> FNLDAEAPAVLSGPPGSFFGFSVEFYRPGTDGVSVLVGAPKANTSQPGVLQGGAVYLCPWGASPTQCTPIEFDSKGSRLLESSLSSSEGEEPVEYKSLQWFGATVRAHGSSILACAPLYSWRTEKEPLSDPVGTCYLSTDNFTRILEYAPCRSDFSWAAGQGYCQGGFSAEFTKTGRVVLGGPGSYFWQGQILSATQEQIAESYYPEYLINLVQGQLQTRQASSIYDDSYLG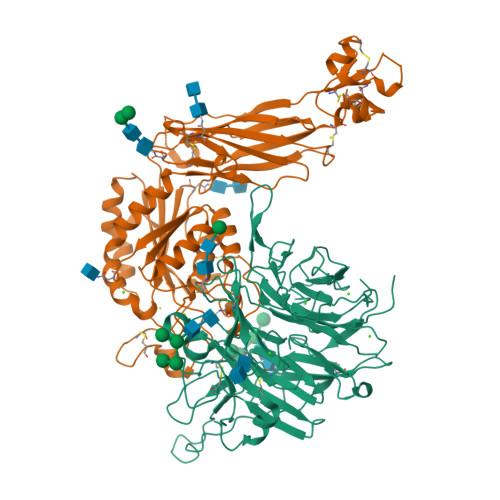YSVAVGEFSGDDTEDFVAGVPKGNLTYGYVTILNGSDIRSLYNFSGEQMASYFGYAVAATDVNGDGLDDLLVGAPLLMDRTPDGRPQEVGRVYVYLQHPAGIEPTPTLTLTGHDEFGRFGSSLTPLGDLDQDGYNDVAIGAPFGGETQQGVVFVFPGGPGGLGSKPSQVLQPLWAASHTPDFFGSALRGGRDLDGNGYPDLIVGSFGVDKAVVYRGRPVV;> QTDENRCLKANAKSCGECIQAGPNCGWCTNSTFLQEGMPTSARCDDLEALKKKGCPPDDIENPRGSKDIKKNKNVTNRSKGTAEKLKPEDITQIQPQQLVLRLRSGEPQTFTLKFKRAEDYPIDLYYLMDLSYSMKDDLENVKSLGTDLMNEMRRITSDFRIGFGSFVEKTVMPYISTTPAKLRNPCTSEQNCTTPFSYKNVLSLTNKGEVFNELVGKQRISGNLDSPEGGFDAIMQVAVCGSLIGWRNVTRLLVFSTDAGFHFAGDGKLGGIVLPNDGQCHLENNMYTMSHYYDYPSIAHLVQKLSENNIQTIFAVTEEFQPVYKELKNLIPKSAVGTLSANSSNVIQLIIDAYNSLSSEVILENGKLSEGVTISYKSYCKNGVNGTGENGRKCSNISIGDEVQFEISITSNKCPKKDSDSFKIRPLGFTEEVEVILQYICECE> GPGGSMKRLRPSDKFFELLGYKPHHVQLAIHRSTAKRRVACLG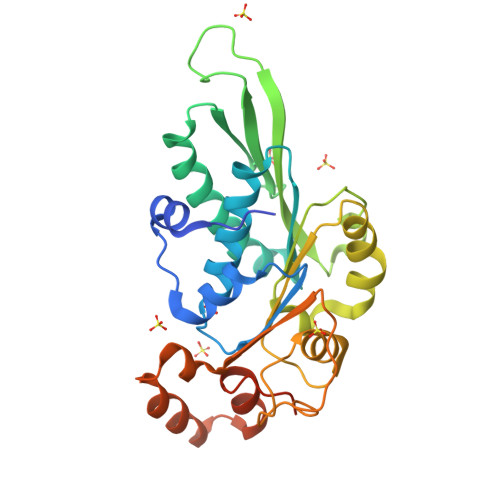RQSGKSEAASVEAVFELFARPGSQGWIIAPTYDQAEIIFGRVVEKVERLAEVFPATEVQLQRRRLRLLVHHYDRPVNAPGAKRVATSEFRGKSADRPDNLRGATLDFVILDEAAMIPFSVWSEAIEPTLSVRDGWALIISTPKGLNWFYEFFLMGWRGGLKEGIPNSGINQTHPDFESFHAASWDVWPERREWYMERRLYIPDLEFRQEYGAEFVSHSGLEHHHHHHHHHH>MNKKIIVMMALLHKEKLIECIYHELENGGTILLLTKNIVVSEISYIGNTYKYFTFNDNHDLISKEDLKGATSKNIAKMIYNWIIKNPQNNKIWSGEPRTQIYFENDLYHTNYNHKCIKDFWNVSTSVGPHI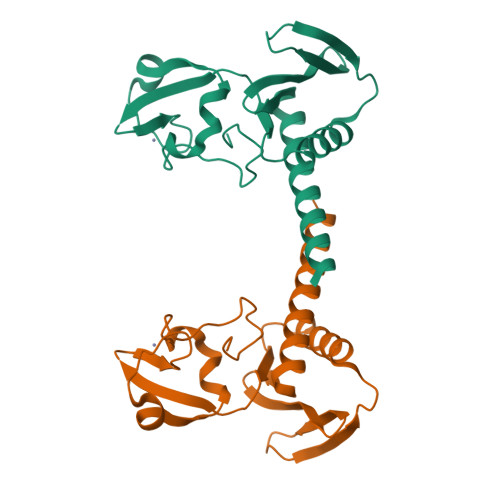FNDRSIWCTKCTSFYPFTNIMSPNIFQ[2x]> NSDVYAQEKQDFVQHFSQIVRVLTEDEMGHPEIGDAIARLKEVLEYNAIGGKYNRGLTVVVAFRELVEPRKQDADSLQRAWTVGWCVEL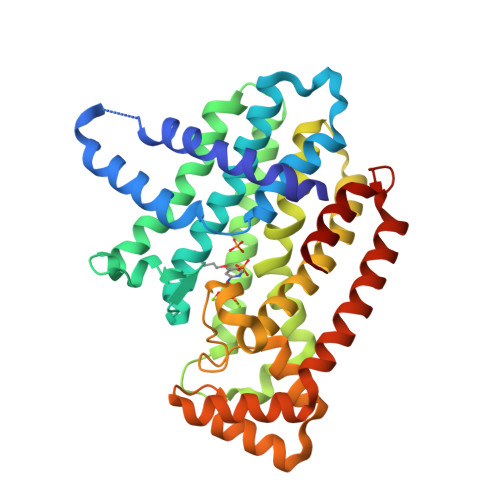LQAFFLVADDIMDSSLTRRGQICWYQKPGVGLDAINDANLLEACIYRLLKLYCREQPYYLNLIELFLQSSYQTEIGQTLDLLTAPQGNVDLVRFTEKRYKSIVKYKTAFYSFYLPIAAAMYMAGIDGEKEHANAKKILLEMGEFFQIQDDYLDLFGDPSVTGKIGTDIQDNKCSWLVVQCLQRATPEQYQILKENYGQKEAEKVARVKALYEELDLPAVFLQYEEDSYSHIMALIEQYAAPLPPAVFLGLARKIYKRRK The phospho-MurNAc-pentapeptide moiety from this intermediate is then transferred to the lipid carrier undecaprenyl phosphate (C55P) at the inner face of the cytoplasmic membrane by the essential integral membrane enzyme MraY, generating the penultimate PG precursor, lipid I. The peripheral membrane enzyme MurG then transfers GlcNAc from UDP-GlcNAc to lipid I, forming lipid II, which contains the basic monomeric unit of PG. MraY is a polytopic membrane protein with ten transmembrane helices. The structure of the enzyme from Aquifex aeolicus revealed that it forms a dimer with most of the monomer–monomer contacts made between the N- and C-terminal helices. Our characterization of this and other related MraY variants supports a model in which MraY is feedback inhibited by the accumulation of flipped lipid II, limiting the synthesis of PG precursors when their supply exceeds the synthetic capacity of PG synthases.

The cryogenic electron microscopy (cryo-EM) structure of the YES complex containing wild-type EcMraY was recently reported, and this methodology was used to obtain the structure of EcMraY(T23P) within the same complex. Focused refinement of MraY alone in the EcMraY(T23P) complex substantially improved the potential lipid density at the MraY dimer interface. As in previous A. aeolicus and E. boltae MraY structures, this electron density fills the hydrophobic cavity found at the MraY dimer interface. However, we uniquely observed this electron density extending into the periplasmic space above the MraY molecules where the environment is more hydrophilic. Although structural refinement could not conclusively identify the lipid within the dimer, the size of the electron density extending into the periplasmic space is consistent with a large head-group such as the disaccharide-pentapeptide found on lipid II. Notably, the T23 residue lies near the dimer interface on the extracytoplasmic side of MraY. We conclude that the T23P substitution generates a hyperactive MraY, leading to elevated lipid II production in cells. Consistent with this possibility, tyrosine at position 21 has an altered conformation in the MraY(T23P) structure in which its hydroxyl group forms a hydrogen bond network with Y227 and K358 on the opposing monomer. Substitutions within these residues were also identified in the screen for hyperactive MraY enzymes, and Y227 is in the periplasmic helix that was found to be altered in the MD analysis upon lipid II binding. Although this result may be affected by the enzyme being stuck in an inhibited state by the phage inhibitor, it suggests that T23P and other changes in MraY may affect the conformational response of the enzyme to lipid II binding rather than the binding event itself.

>MLVWLAEHLVKYYSGFNVFSYLPFRAIVSLLTALFISLWMGPRMIAHLQKLSFGQVVRNDGPESHFSKRGTPTMGGIMILTAIVISVLLWAYPSNPYVWCVLVVLVGYGVIGFVDDYRKVVRKDTKGLIARWKYFWMSVIALGVAFALYLAGKDTPATQLVVPFFKDVMPQLGLFYILLAYFVIVGTGNAVNLTDGLDGLAIMPTVFVAGGFALVAWATGNMNFASYLHIPYLRHAGELVIVCTAIVGAGLGFLWFNTYPAQVFMGDVGSLALGGALGIIAVLLRQEFLLVIMGGVFVVETLSVILQVGSFKLRGQRIFRMAPIHHHYELKGWPEPRVIVRFWIISLMLVLIGLATLKVR[2x]>[3x]MSFFHASQRDALNQSLAEVQGQINVSFEFFPPRTSEMEQTLWNSIDRLSSLKPK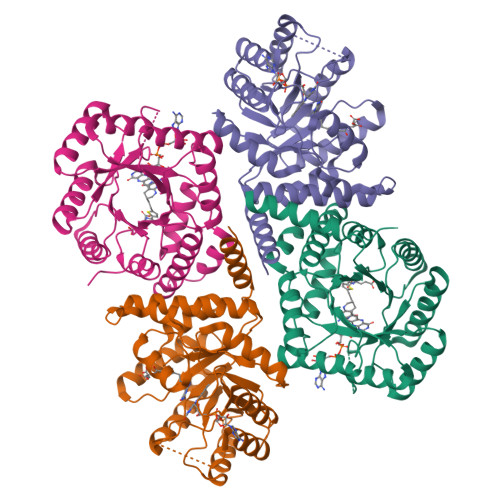FVSVTYGANSGERDRTHSIIKGIKDRTGLEAAPHLTCIDATPDELRTIARDYWNNGIRHIVALRGDLPPGSGKPEMYASDLVTLLKEVADFDISVAAYPEVHPEAKSAQADLLNLKRKVDAGVNRAITQFFFDVESYLRFRDRCVSAGIDVEIIPGILPVSNFKQAKKFADMTNVRIPAWMAQMFDGLDDDAETRKLVGANIAMDMVKILSREGVKDFHFYTLNRAEMSYAICHTLGVRPGLLEHHHHHH>NIEGVFRKSFPDLAGETLLDSFNCAWVEGSALKQGYLFITPHWLCFQSTLAAAHFSIEYDEIKDIIKSKSVKMFENAIEVKTHLNDTIFLTNFLQRDQAYSALMSQW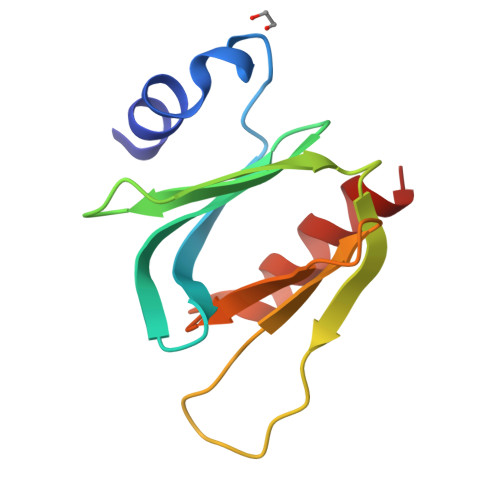LKQ[2x]>GMDAGRGAEHDEAVTSDDSASVEVPRRATPADAATVAQMLHDFNTEFGAPTPGTDELASRLSHLLAGED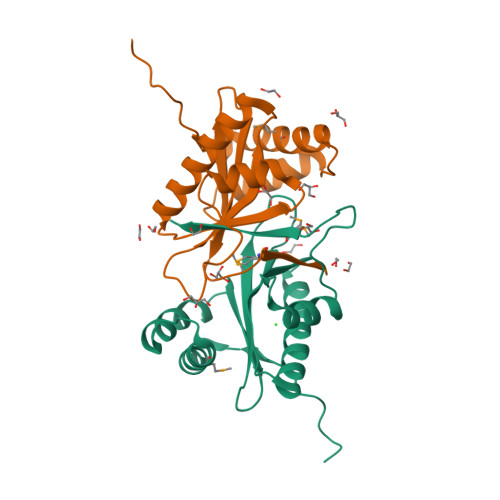VVVLLAGEPPTGLAVLSFRPNVWYPGPVAILDELYVRPGRRGHRLGSALLAASCGLVRSRGGALLEINVDGEDTDARRFYEARGFTNTEPNGTEPMLYYYREL[2x]>[3x]GPLGSAVSLVQAQTNARAIAAMKNSIQATNRAVF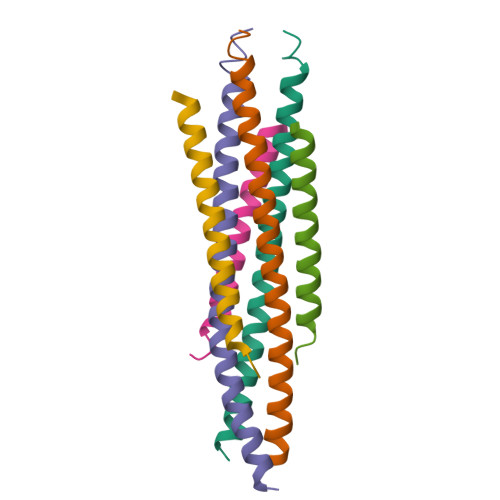EVKEGTQRLAIAVQAIQDHINTIMNTQLN;>[3x]NMSSGGRGGIDISTELSKVNASLQNTVKYIKESNHQLQSVIVNSKIGA> SWCLSVHQPWASLLVRGIKRVEGRSWYTPHRGRLWIAATAKKPSPQEVSELQATYRLLRGKDVEFPNDYPSGCLLGCVDLIDCLSQKQFKEQFPDISQESDSPFVFIC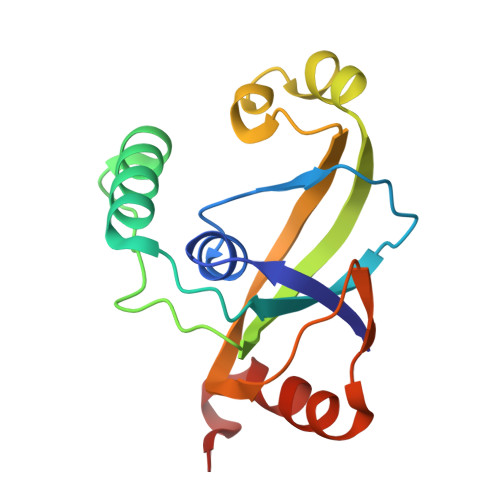KNPQEMVVKFPIKGNPKIWKLDSKIHQGAKKGLMKQNKAV>GPMAEKLNFEELNSMQRYSQFAVFRAIPGALGSDRAEIVAQAQSFFDGLETAGKVEVRGIYDLAGCRAEADFMIWWIAEEFEEIQAAFARFRRETVLGQVSEVAWLGNSLHRPAEFNRSHLPSFIMGEIPGDWITVYPFVRSYDWYIMDPQKRRKILAEHGQAARDFPDVRANTVPAFALGDYEYMLAFEAPRLDRIVDLMH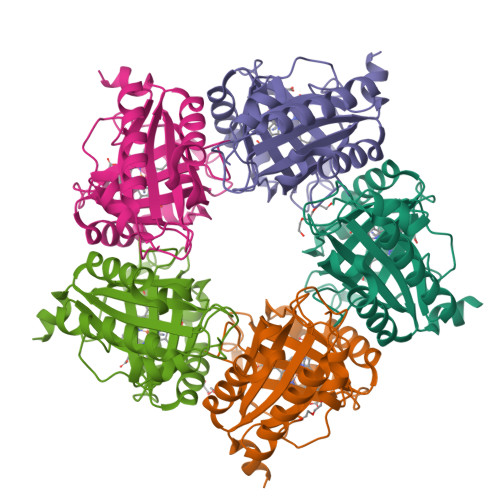KMRYTEARLHVREETPFFTGRRVSEVSELVNVLPG[5x]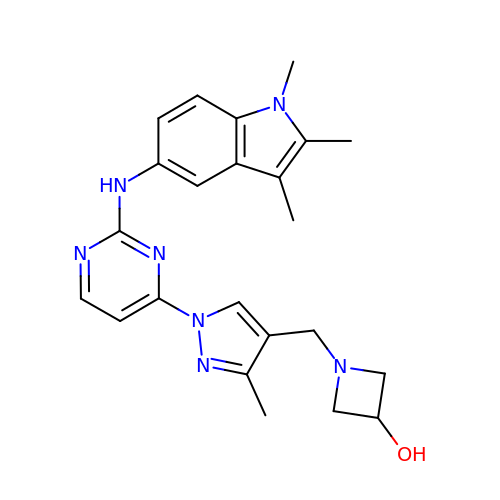1-[(3-methyl-1-{2-[(1,2,3-trimethyl-1H-indol-5-yl)amino]pyrimidin-4-yl}-1H-pyrazol-4-yl)methyl]azetidin-3-ol | C23 H27 N7 O | WVDKJJLIGILVRJ-UHFFFAOYSA-N> KSSNEATNITPKHNMKAFLDELKAENIKKFLYNFTQIPHLAGTEQNFQLAKQIQSQWKEFGLDSVELAHYDVLLSYPNKTHPNYISIINEDGNEIFNTSLFEPPPPGYENVSDIVPPFSAF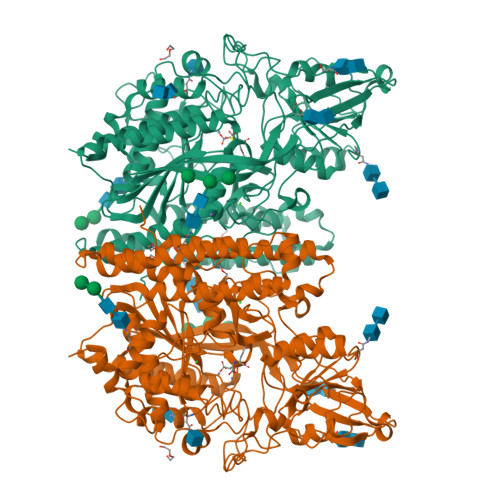SPQGMPEGDLVYVNYARTEDFFKLERDMKINCSGKIVIARYGKVFRGNKVKNAQLAGAKGVILYSDPADYFAPGVKSYPDGWNLPGGGVQRGNILNLNGAGDPLTPGYPANEYAYRRGIAEAVGLPSIPVHPIGYYDAQKLLEKMGGSAPPDSSWRGSLKVPYNVGPGFTGNFSTQKVKMHIHSTNEVTRIYNVIGTLRGAVEPDRYVILGGHRDSWVFGGIDPQSGAAVVHEIVRSFGTLKKEGWRPRRTILFASWDAMEFGLLGSTEWAEENSRLLQERGVAYINADSSIEGNYTLRVDCTPLMYSLVHNLTKELKSPDEGFEGKSLYESWTKKSPSPEFSGMPRISKLGSGNDFEVFFQRLGIASGRARYTKNWETNKFSGYPLYHSVYETYELVEKFYDPMFKYHLTVAQVRGGMVFELANSIVLPFDCRDYAVVLRKYADKIYSISMKHPQEMKTYSVSFDSLFSAVKNFTEIASKFSERLQDFDKSNPIVLRMMNDQLMFLERAFIDPLGLPDRPFYRHVIYAPSSHNKYAGESFPGIYDALFDIESKVDPSKAWGEVKRQIYVAAFTVQAAAETLSEVA For promoter-specific transcription, RNAP and general transcription factors (GTFs) are recruited to the promoter DNA to form the pre−initiation complex (PIC). In this study, we determined the X-ray structure of TFEα and the cryo-EM structures of three forms of archaeal RNAP, including the apo-form, RNAP–TFEα binary complex, and RNAP–TFEα–DNA ternary complex. The structures reveal that direct binding of TFEα can shift the clamp conformation from a closed conformation to an open conformation. Our results support the universally conserved mechanisms of transcription initiation in all three domains of life by showing that direct binding of TFEα, a conserved GTF in archaeal-eukaryal RNAP systems, can open the clamp of the stalk-containing RNAPs.

After screening derivatives of TFEα, we found that the 13 kDa fragment Pfu TFEα (TFEαΔZRD, 1–110 amino acid residues) was crystallized. The structure was solved by a single wavelength anomalous dispersion (SAD) at 3.2 Å and the resolution of the structure was improved to 2.6 Å with a native crystal. There were eight molecules in the asymmetric unit of the SAD structure and two molecules in the asymmetric unit of the native structure. The TFEαΔZRD structure consists of the N-terminal eWHD (residues 5–86) and a long α-helix (α5) that connects the eWHD and the ZRD. The eWHD structure is similar with the X-ray crystal structures of the eWHD of Sso TFEα15 and the eWHD of human TFIIEα23. Superposition of the globular part of the eWHD from the 10 crystallographically independent structures (average root-mean-square deviation in α-carbon positions are 0.369–0.589 Å over residues 8–62) reveal flexibilities in the wing and the α5 linker. The conformation of the wing can change about 24° (~13 Å), and the α5 can be bent at ~21° (~12 Å) for the eWHD. These results show a potential structural adaptability of TFEα during the transcription initiation process.

>[2x]MGRDKKNTALLDIARDIGGDEAVEVVKALEKKGEATDEELAELTGVRVNTVRKILYALYDAKLATFRRVRDDETGWYYYYWRIDTKRLPEVIRTRKLQELEKLKQMLQEETSETYYHCGTPGHPKLTFDEAFEYGFQCPICGEILYEYDNSKIIEELKKRIEELEIELGLRSPPKEEKPKKATRRKKSRSGKKKK>[5x]MTITYTSQVANARLGSFSRLLLCWRGSIYKLLYGEFLIFLLCYYIIRFIYRLALTEEQQLMFEKLTLYCDSYIQLIPISFVLGFYVTLVVTRWWNQYENLPWPDRLMSLVSGFVEGKDEQGRLLRRTLIRYANLGNVLILRSVSTAVYKRFPSAQHLVQAGFMTPAEHKQLEKLSLPHNMFWVPWVWFANLSMKAWLGGRIRDPILLQSLLNEMNTLRTQCGHLYAYDWISIPLVYTQVVTVAVYSFFLTCLVGRQFLNPAKAYPGHELDLVVPVFTFLQFFFYVGWLKVAEQLINPFGEDDDDFETNWIVDRNLQVSLLAVDEMHQDLPRMEPDMYWNKPEPQP

Bestrophin-1 (Best1) and bestrophin-2 (Best2) are two members of the bestrophin family of calcium (Ca2+)-activated chloride (Cl−) channels with critical involvement in ocular physiology and direct pathological relevance. The bestrophins are a family of Ca2+-activated anion channels consisting of four members (Best1–4) in mammals. The overall architecture of hBest1 and hBest2 resembles the pentameric assembly previously shown by KpBest, cBest1 and bBest2, and retains the two landmark permeation constrictions, the neck and aperture, in the ion conducting pathway. Ample electrophysiological evidence indicates that the neck and aperture serve as dual Ca2+-dependent channel “gates”, as disrupting either of them partially impairs Ca2+-dependence while disrupting both makes the channel completely Ca2+-independent.

To further investigate the structural significance of the AS, we generated hBest11–345 and bBest21–345, and solved their structures in the presence of 5 mM Ca2+ at 2.4 Å and 1.9 Å, respectively. Remarkably, both structures exhibited 100% of particles with a fully open neck, in sharp contrast to the only ~10% particles with partially or fully open neck in WT hBest1 and hBest2, respectively. Although a fully open neck was observed in hBest11–345, it is unclear whether or how the neck in hBest1, in the presence of the AS, adapts to the fully open conformation in physiological conditions. Remarkably, hBest11–345 and hBest21–345 were indistinguishable, both displaying robust leak currents with similar amplitudes in the absence of Ca2+ and significantly increased currents with similar amplitudes at 1 μM Ca2+ compared to the respective FL channels (using two-tailed unpaired Student t test), which is consistent with the 100% fully open neck in their structures. Remarkably, removing the AS from hBest1 and hBest2 results in truncation mutants that both exhibit a fully open neck in 100% of Ca2+-bound particles in cryo-EM and conduct indistinguishable and significantly elevated currents in patch clamp, while swapping the AS between hBest1 and hBest2 results in chimeric mutants with exchanged channel activities.> MAAHHRQNTAGRRKVQVSYVIRDEVEKYNRNGVNALQLDPALNRLFTAGRDSIIRIWSVNQHKQDPYIASMEHHTDWVNDIVLCCNGKTLISASSDTTVKVWNAHKGFCMSTLRTHKDYVKALAYAKDKELVASAGLDRQIFLWDVNTLTALTASNNTVTTSSLSGNKDSIYSLAMNQLGTIIVSGSTEKVLRVWDPRTCAKLMKLKGHTDN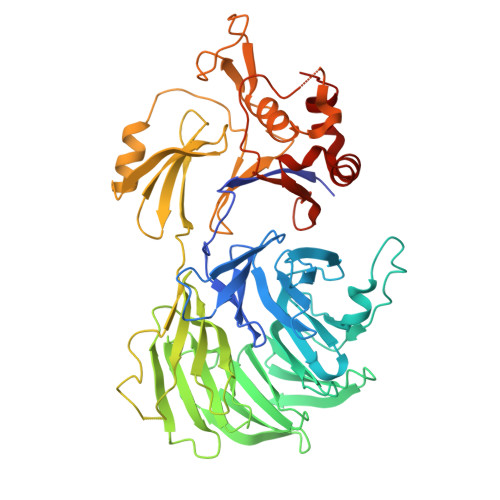VKALLLNRDGTQCLSGSSDGTIRLWSLGQQRCIATYRVHDEGVWALQVNDAFTHVYSGGRDRKIYCTDLRNPDIRVLICEEKAPVLKMELDRSADPPPAIWVATTKSTVNKWTLKGIHNFRASGDYDNDCTNPITPLCTQPDQVIKGGASIIQCHILNDKRHILTKDTNNNVAYWDVLKACKVEDLGKVDFEDEIKKRFKMVYVPNWFSVDLKTGMLTITLDESDCFAAWVSAKDAGFSSPDGSDPKLNLGGLLLQALLEYWPRTHVNPMDEEENEVNHVNGEQENRVQKGNGYFQVPPHTPVIFGEAGGRTLFRLLCRDSGGETESMLLNETVPQWVIDITVDKNMPKFN In the Firmicutes phylum, GpsB is a membrane associated protein that coordinates peptidoglycan synthesis with cell growth and division. GpsB is a DivIVA-like protein that is highly conserved in Firmicutes. The full-length Sa GpsB is a relatively small protein of 114 residues. Its N-terminal domain homodimerizes as a coiled-coil, while its smaller C-terminal domain homotrimerizes, forming a hexamer as the biological unit. Dimerization of the N-terminal domain is facilitated by a pattern of nonpolar residues every three to four residues, promoting the formation of a hydrophobic core in the coiled-coil. This N-terminal domain is partitioned into three regions: a relatively short α-helix with approximately two turns (residues 10–16), a second longer α-helix (residues 28–70) that forms a coiled-coil, and an amphipathic 10-residue loop (residues 17–27) that links these two helices and intertwines with the adjacent protomer, ‘capping’ GpsB.

Using X-ray crystallography, we solved the structure of the N-terminal domain (residues 1–70) of Sa GpsB at 1.95 Å resolution in the P21 space group, with four monomers per asymmetric unit forming two dimers (dimers A and B). The overall structure of GpsB is similar to previously determined GpsB orthologs (Rismondo et al., 2016; Cleverley et al., 2019) and retains the same fold of DivIVA, though it shares much less sequence similarity. The most unique structural feature of Sa GpsB is a hinge forming at the midpoint of its N-terminal domain that causes each protomer to bend, adopting pitch angles (θ) of 137–140° (dimer A) and 156–166° (dimer B). In contrast, GpsB protomers from Lm, Bs, Sp, and Sa DivIVA are almost linear (θ=167–179°) and practically indistinguishable when superimposed. We find that there is a 3-amino acid insertion in the Sa GpsB sequence where the helicity is disrupted and that a cluster of four Met residues (Met45, Met48) are interlocked at the dimer interface at this position (dotted rectangle). These Met residues are only found in Staphylococci and take the place of an aromatic Tyr or Phe present in other orthologs, which normally stabilize the core via π stacking interactions. While the 3-amino acid insertion likely disrupts the continuity of the coiled-coil, methionine is one of the most flexible aliphatic amino acids and may further contribute to the conformational flexibility. Experiments using solution state NMR spectroscopy further support the notion of intrinsic conformational heterogeneity, suggesting it is a bona fide structural feature rather than a crystallization artifact. By extending the asymmetric unit, we found each GpsB dimer coordinates two others in a head-to-head arrangement. This involves the insertion of Arg and Lys residues from the membrane-binding loop into the PBP-binding site from the adjacent GpsB protomer, mimicking the binding mode observed between PBP mini-domains and GpsB in orthologous structures, such as Bs PBP1 (Cleverley et al., 2019).

>HMSDVSLKLSAKDIYEKDFEKTMARGYRREEVDAFLDDIIADYQKMADMNNEVVKLSEENHKLKKELEELR[4x]> HHHHHHMGIEWIIRRSVANRFLVLMGALFLSIWGTWTIINTPVDALPDLSDVQVIIKTSYPGQAPQIVENQVTYPLTTTMLSVPGAKTVRGFSQFGDSYVYVIFEDGTDPYWARSRVLEYLNQVQGKLPAGVSAELGPDATGVGWIYEYALVDRSGKHDLADLRSLQDWFLKYELKTIPDVAEVASVGGVVKEYQVVIDPQRLAQYGISLAEVKSALDASNQEAGGSSIELAEAEYMVRASGYLQTLDDFNHIVLKASENGVPVYLRDVAKVQIGPEMRRGIAELNGEGEVAGGVVILRSGKNAREVIAAVKDKLETLKSSLPEGVEIVTTYDRSQLIDRAIDNLSGKLLEEFIVVAVVCALFLWHVRSALVAIISLPLGLCIAFIVMHFQGLNANIMSLGGIAIAVGAMVDAAIVMIENAHKRLEEWQHQHPDATLDNKTRWQVITDASVEVGPALFISLLIITLSFIPIFTLEGQEGRLFGPLAFTKTYAMAGAALLAIVVIPILMGYWIRGKIPPESSNPLNRFLIRVYHPLLLKVLHWPKTTLLVAALSVLTVLWPLNKVGGEFLPQINEGDLLYMPSTLPGISAAEAASMLQKTDKLIMSVPEVARVFGKTGKAETATDSAPLEMVETTIQLKPQEQWRPGMTMDKIIEELDNTVRLPGLANLWVPPIRNRIDMLSTGIKSPIGIK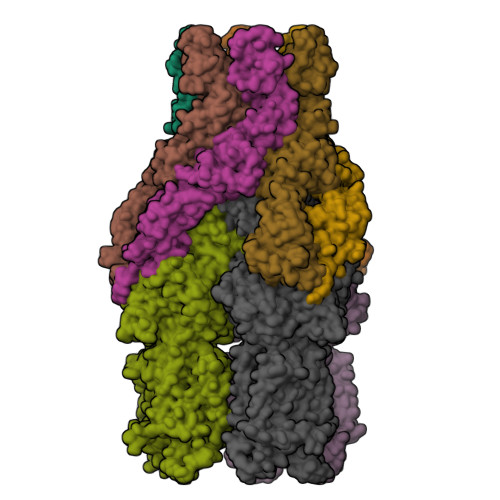VSGTVLADIDAMAEQIEEVARTVPGVASALAERLEGGRYINVEINREKAARYGMTVADVQLFVTSAVGGAMVGETVEGIARYPINLRYPQSWRDSPQALRQLPILTPMKQQITLADVADIKVSTGPSMLKTENARPTSWIYIDARDRDMVSVVHDLQKAIAEKVQLKPGTSVAFSGQFELLERANHKLKLMVPMTLMIIFVLLYLAFRRVGEALLIISSVPFALVGGIWLLWWMGFHLSVATGTGFIALAGVAAEFGVVMLMYLRHAIEAVPSLNNPQTFSEQKLDEALYHGAVLRVRPKAMTVAVIIAGLLPILWGTGAGSEVMSRIAAPMIGGMITAPLLSLFIIPAAYKLMWLHRHRVRK;>[2x]MKKIALIIGSMIAGGIISAAGFTWVAKAEPPAEKTSTAERKILFWYDPMYPNTRFDKPGKSPFMDMDLVPKYADEESSASGVRIDPTQTQNLGVKTATVTRGPLTFAQSFPANVSYNEYQYAIVQARAAGFIDKVYPLTVGDKVQKGTPLLDLTIPDWVEAQSEYLLLRETGGTATQTEGILERLRLAGMPEADIRRLIATQKIQTRFTLKAPIDGVITAFDLRAGMNIAKDNVVAKIQGMDPVWVTAAIPESIAWLVKDASQFTLTVPARPDKTLTIRKWTLLPGVDAATRTLQLRLEVDNADEALKPGMNAWLQLNTASEPMLLIPSQALIDTGSEQRVITVDADGRFVPKRVAVFQASQGVTALRSGLAEGEKVVSSGLFLIDSEANISGALERMRSESATHAHHHHHHH> APGDPCDEPLVSGLPHVAFSSSSSISGSYS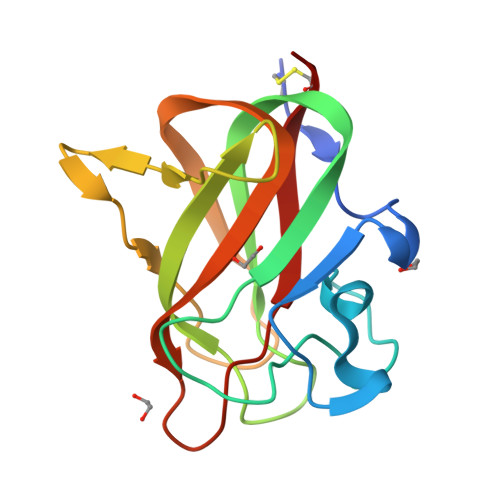PGYAKINKRGGAGGWSPSDSDHYQWLQVDFGNRKQISAIATQGRYSSSDWVTQYRMLYSDTGRNWKPYHQDGNIWAFPGNINSDGVVRHELQHPIIARYVRIVPLDWNGEGRIGLRIEVYGCAA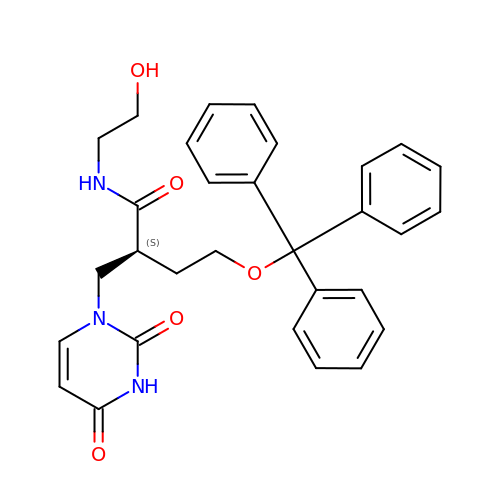(2S)-2-[(2,4-dioxopyrimidin-1-yl)methyl]-N-(2-hydroxyethyl)-4-trityloxy-butanamide | C30 H31 N3 O5 | POOIRAMVDDLAIT-QHCPKHFHSA-N The HCV NS3/4A protease – a chymotrypsin-like serine protease – is a prime therapeutic target that cleaves four known sites along the virally encoded polyprotein. The NS3/4A protease also hydrolyzes two human proteins, TRIF and MAVS, which are part of the innate immune system, thereby confounding the innate immune response to viral infection. In this study, we report that four chemically representative protease inhibitors – telaprevir, danoprevir, vaniprevir and MK-5172 – exhibit distinct susceptibilities to the protease variants R155K, A156T and D168A. To elucidate the underlying mechanism by which chemically diverse inhibitors bind to the wild-type protease and drug-resistant variants, crystal structures were determined for 16 inhibitor-protease complexes. These complexes include wild-type protease and resistant variants R155K, D168A and A156T each bound to telaprevir, danoprevir, vaniprevir and MK-5172, with resolutions ranging from 1.10–2.50 Å; S139A protease variants were used except for telaprevir, which requires covalent bond formation with the serine 139 for efficient binding.

Telaprevir potency was slightly better against D168A relative to the wild type, while danoprevir, vaniprevir and MK-5172 lost 100- to 1000-fold potency against D168A. Among the macrocyclic drugs, danoprevir and MK-5172 retained higher activities against D168A (D168A IC50 = 48 nM and 13 nM, respectively) relative to vaniprevir (D168A IC50>400 nM). Unlike in the danoprevir and vaniprevir complexes with wild type, in the MK-5172-wild-type complex the P2 quinoxaline moiety did not stack on R155 and interacted less with D168 and the electrostatic network involving these residues. Thus, the single-site mutations R155K and D168A only caused very subtle changes in the MK-5172 binding conformations. This subtle effect is reflected in the small loss of potency against the R155K variant; however, MK-5172 exhibited 100-fold lower potency against the D168A variant, likely due to less extensive interactions with D81 and K136 relative to wild-type and R155K. Overall, analysis of the four crystal structures explains MK-5172's significantly retained potency against R155K and D168A as well as its loss of potency against the A156T variant due to the rigidity of the macrocycle. Unlike other inhibitors, MK5172 does not directly interact with R155 and D168, which mutate to confer multi-drug resistance. This unique binding mode of MK-5172 explains its significantly greater potency against R155K and D168A variants compared to other inhibitors.

>GSHMASMKKKGSVVIVGRINLSGDTAYAQQTRGEEGCQETSQTGRDKNQVEGEVQIVSTATQTFLATSINGVLWTVYHGAGTRTIASPKGPVTQMYTNVDKDLVGWQAPQGSRSLTPCTCGSSDLYLVTRHADVIPVRRRGDSRGSLLSPRPISYLKGSSGGPLLCPAGHAVGIFRAAVCTRGVAKAVAFIPVESLETTMRSP[4x]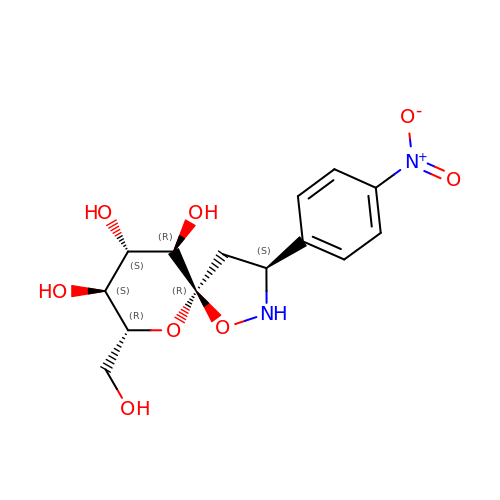(3S,5R,7R,8S,9S,10R)-7-(hydroxymethyl)-3-(4-nitrophenyl)-1,6-dioxa-2-azaspiro[4.5]decane-8,9,10-triol | C14 H18 N2 O8 | FYUHHVCQKVTVLN-GMDXDWKASA-N> FDSFWFVQQWPPAVCSFQKSGSCPGSGLRTFTIHGLWPQQSGTSLTNCPGSPFDITKISHLQSQLNTLWPNVLRANNQQFWSHEWTKHGTCSESTFNQAAYFKLAVDMRNNYDIIGALRPHAAGPNGRTKSRQAIKGFLKAKFGKFPGLRCRTDPQTKVSYLVQVVACFAQDGSTLIDCT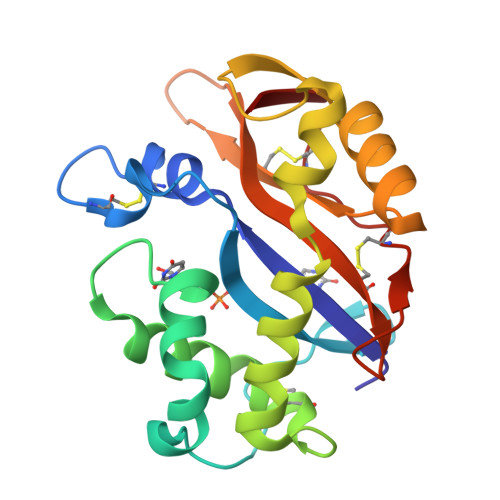RDTCGANFIF>[2x]GPGSPQSDMNNIKPLEGVKILDLTRVLAGPFATMNLGDLGAEVIKVERPGAGDDTRTWGPPFVGTESTYYLSVNRNKKSIAVNIKDPKGVKIIKELAAVCDVFVENYVPGKLSAMGLGYEDIDEIAPHIIYCSITGYGQTGPISQRAGYDAVASAVSGLMHITGPENGDPVRPGVAMTDLATGLYAYGAIMAGLIQKYKTGKGLFIDCNLLSSQVACLSHIAANYLIGQKEAKRWGTAHGSIVPYQAFK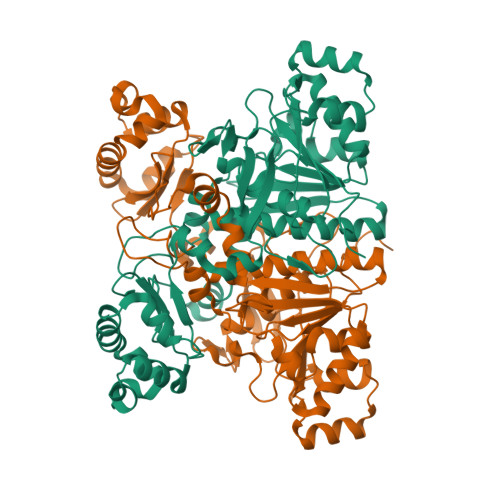TKDGYIVVGAGNNQQFATVCKILDLPELIDNSKYKTNHLRVHNRKELIKILSERFEEELTSKWLYLFEGSGVPYGPINNMKNVFAEPQVLHNGLVMEMEHPTVGKISVPGPAVRYSKFKMSEARPPPLLGQHTTHILKEVLRYDDRAIGELLSAGVVDQHETH> MFALRTAARPAARSVGATRNYATL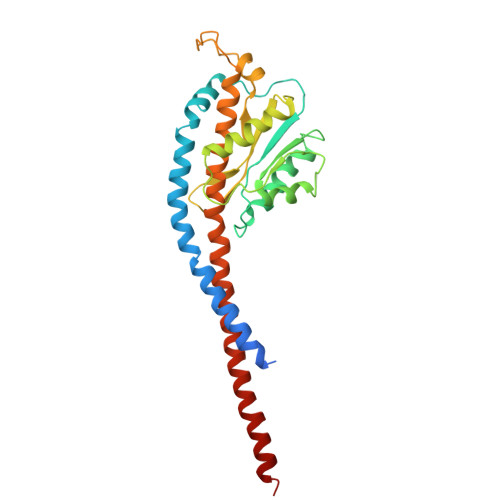REIEMRLKSIKNIEKITNTMKIVASTKLGKAQRAMATSKVYNEASEKVFENSETAVPENIEKRLWVVVSSDKGLCGSIHSQLARTVRRKLLDFESGEKLIDIVAVGEKIKAQLGRSNPEQMRLSFGGTGKEAPTFEEAAHIADEILALDTQYDDIEIVYNKVLSGISFEPIMKESYSAKAIEDAPKFGQYELEDDVVKNLADFSLANTIYAAMAEGHAAEISARRNAMDNASKNASDMINKYSILYNRTRQAVITNELVDIITGASSLE1-[(4-fluorophenyl)amino]thiourea | C7 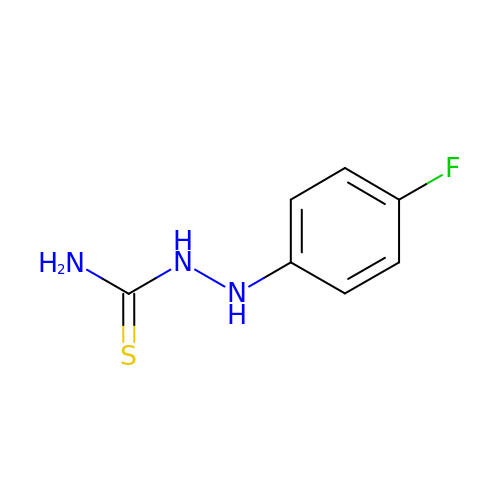H8 F N3 S | KQNHAXWTVPXGMP-UHFFFAOYSA-N> GSFTARPSSSMADFRKFFAKAKHIVIISGAGVSAESGVPTFRGAGGYWRKWQAQDLATPLAFAHNPSRVWEFYHYRREVMGSKEPNAGHRAIAECETRLGKQGRRVVVITQNIDELHRKAGTKNLLEIHGSLFKTRCTSCGVVAENYKSPICPALSGKGAPEPGTQDASIPVEKLPRCEEAGCGGLLRPHVVWFGENLDPAILEEVDRELAHCDL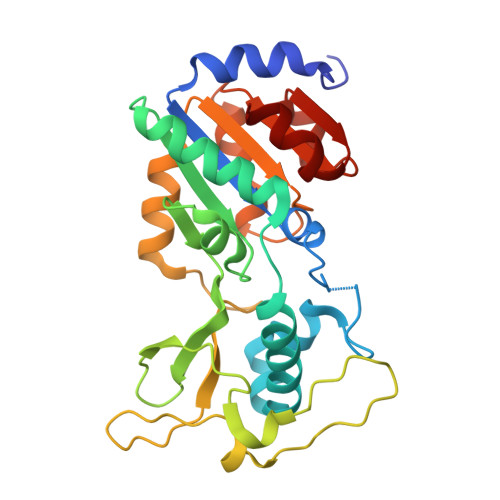CLVVGTSSVVYPAAMFAPQVAARGVPVAEFNTETTPATNRFRFHFQGPCGTTLPEALA[2-({4-[(2-amino-4-oxo-4,7-dihydro-3H-pyrrolo[2,3-d]pyrimidin-5-yl)methyl]benzene-1-carbonyl}amino)phenyl]acetic 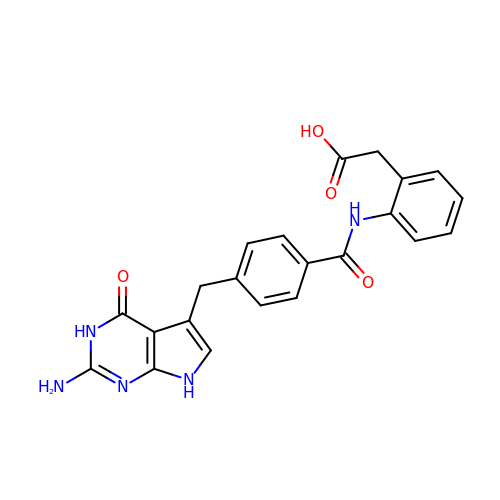acid | C22 H19 N5 O4 | NCEMLZMBZDJVMM-UHFFFAOYSA-N>[2x]GPDSENGVGDAELRERLRQCEETIEQLRAENQELKRKLNILTRPSGILVNDTKLDGPILQILFMNNAISKQYHQEIEEFVSNLVKRFEEQQKNDVEKTSFNLLPQPSSIVLEEDHKVEESCAIKNNKEAFSVVGSVLYFTNFCLDKLGQPLLNENPQLSEGWEIPKYHQVFSHIVSLEGQEIQVKAKRPKPHCFNCGSEEHQMKDCPMPRNAARISEKRKEYMDACGEANNQNFQQRYHAEEVEERFGRFKPGVISEELQDALGVTDKSLPPFIYRMRQLGYPPGWLKEAELENSGLALYD;>[2x]GPDSMADAFGDELFSVFEGDSTTAAGTKKDKEKDKGKWKGPPGSADKAGKRFDGKLQSESTNNGKNKRDVDFEGTDEPIFGKKPRIEESITEDLSLADLMPRVKVQSVETVEGCTHEVALPAEEDYLPLKPRVGKAAKEYPFILDAFQREAIQCVDNNQSVLVSAHTSAGKTVCAEYAIALALREKQRVIFTSPIKALSNQKYREMYEEFQDVGLMTGDVTINPTASCLVMTTEILRSMLYRGSEVMREVAWVIFDEIHYMRDSERGVVWEETIILLPDNVHYVFLSATIPNARQFAEWICHLHKQPCHVIYTDYRPTPLQHYIFPAGGDGLHLVVDENGDFREDNFNTAMQVLRDAGDLAKGDQKGRKGGTKGPSNVFKIVKMIMERNFQPVIIFSFSKKDCEAYALQMTKLDFNTDEEKKMVEEVFSNAIDCLSDEDKKLPQVEHVLPLLKRGIGIHHGGLLPILKETIEILFSEGLIKALFATETFAMGINMPARTVL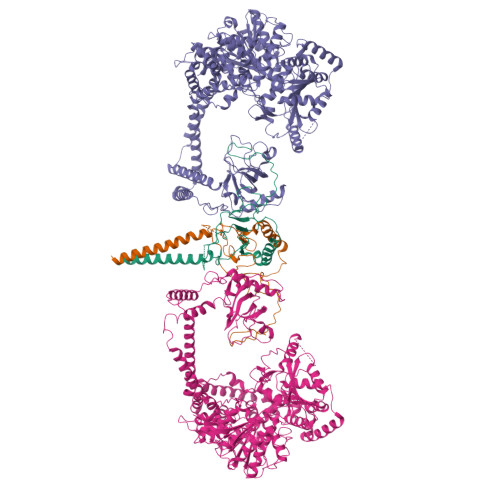FTNARKFDGKDFRWISSGEYIQMSGRAGRRGMDDRGIVILMVDEKMSPTIGKQLLKGSADPLNSAFHLTYNMVLNLLRVEEINPEYMLEKSFYQFQHYRAIPGVVEKVKNSEEQYNKIVIPNEESVVIYYKIRQQLAKLGKEIEEYIHKPKYCLPFLQPGRLVKVKNEGDDFGWGVVVNFSKKSNVKPNSGELDPLYVVEVLLRCSKESLKNSATEAAKPAKPDEKGEMQVVPVLVHLLSAISSVRLYIPKDLRPVDNRQSVLKSIQEVQKRFPDGIPLLDPIDDMGIQDQGLKKVIQKVEAFEHRMYSHPLHNDPNLETVYTLCEKKAQIAIDIKSAKRELKKARTVLQMDELKCRKRVLRRLGFATSSDVIEMKGRVACEISSADELLLTEMMFNGLFNDLSAEQATALLSCFVFQENSSEMPKLTEQLAGPLRQMQECAKRIAKVSAEAKLEIDEETYLSSFKPHLMDVVYTWATGATFAHICKMTDVFEGSIIRCMRRLEELLRQMCQAAKAIGNTELENKFAEGITKIKRDIVFAASLYL>MPSETPQAEVGPTGCPHRSGPHSAKGSLEKGSPEDKEAKEPLWIRPDALSRCTWQLGRPASESPHHHTAPAKSPKILPDILKKIGDTPMVRINKIGKKFGLKCELLAKCEFFNAGGSVKDRISLRMIEDAERDGTLKPGDTIIEPTSGNTGIGLALAAAVRGYRCIIVMPEKMSSEKVDVLRALGAEIVRTPTNARFDSPESHVGVAWRLKNEIPNSHILDQYRNASNPLAHYDTTADEILQQCDGKLDMLVASVGTGGTITGIARKLKEKCPGCRIIGVDPEGSILAEPEELNQTEQTTYEVEGIGYDFIPTVLDRTVVDKWFKSNDEEAFTFARMLIAQEGLLCGGSAGSTVAVAVKAAQELQEGQRCVVILPDSVRNYMTKFLSDRWMLQKGFLKEEDLTEKKPW[6x]

CBS catalyzes the condensation of homocysteine and serine (or cysteine) leading to formation of cystathionine and H2O (or H2S). The human enzyme is a 551-amino acid protein with a central catalytic domain, harboring a pyridoxal 5′-phosphate (PLP) cofactor, flanked by a C-terminal domain with a binding site for the allosteric positive regulator s-adenosyl-l-methionine (AdoMet) and an N-terminal domain, harboring a hexacoordinate heme with C52 and H65 as endogenous Fe ligands. While the enzyme is fully active when the heme is in the oxidized state, reduction to the ferrous state negatively impacts enzyme activity, possibly through a ligand exchange mechanism involving the replacement of C52 by a yet unknown neutral ligand. Classical homocystinuria (OMIM #236200) is an inborn error of metabolism associated with mutations in the CBS gene.

The 146 C>T transition in exon 1 of the CBS gene generates the clinically relevant p.P49L variant, identified in patients with classical homocystinuria. The crystallographic structure of a truncated version of CBS p.P49L, devoid of the C-terminal AdoMet binding domain, reveals no major differences at the level of the PLP catalytic site with respect to the WT but slightly increased protein flexibility in the heme surroundings. There are six molecules in the asymmetric unit corresponding to a Matthews coefficient of 2.31 Å3·Da−1 and a solvent content of approximately 47%. The structure was refined to 2.80 Å resolution with Rcryst of 18.2% and Rfree of 22.1%. The final model comprises the residues from R45 to E400 (in chain D), 6 hemes, 6 PLP molecules, 3 sodium ions, and 185 water molecules. The hemes are axially bridged by C52 and H65 and the PLP moieties covalently linked to the polypeptide chain through K119. Within the obtained resolutions, the structures display highly conserved features, particularly inspecting the PLP binding pocket with the cofactor covalently bound to K119, the heme ligands C52 and H65, α-helix 8 (responsible for the heme-PLP communication), the R266 residue forming a salt-bridge with C52, and the flexible loop where the mutated P49 residue is located. We thus looked in greater detail at the heme binding region and found in CBS p.P49L an increased flexibility of the loop surrounding the C52 ligand, which expands to the regions between the C52 and H65 ligands and even after the latter residue. The p.P49L structure therefore displays a higher flexibility in the region harboring both heme ligands, which provides a possible structural basis for the proposed slower rebinding of the endogenous C52/X ligands upon CO dissociation, thereby accounting for the increased affinity of CBS p.P49L for CO. Notably, the CO affinity, herein measured for the first time in a CBS variant, is markedly increased (≥50-fold) in CBS p.P49L with respect to the WT enzyme.> ASHSRKFLDVRSEEELLSCIKKETEAGKLPPNVAAGMEELYQNYRNAVIESGNPKADEIVLSNMTVALDRILLDVEDPFVFSSHHKAIREPFDYYIFGQNYIRPLIDFGNSFVGNLSLFKDIEEKLQQGHNVVLISNHQTEADPAIISLLLEKTNPYIAENTIFVAGDRVLADPL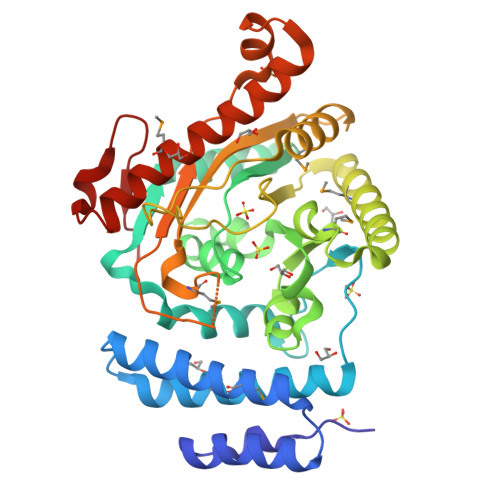CKPFSIGRNLICVYSKKHMFDIPELTETKRKANTRSLKEMALLLRGGSQLIWIAPSGGRDRPDPSTGEWYPAPFDASSVDNMRRLIQHSDVPGHLFPLALLCHDIMPPPSQVEIEIGEKRVIAFNGAGLSVAPEISFEEIAATHKNPEEVREAYSKALFDSVAMQYNVLKTAISGKQGLGASTADVSLSQPW[(2~{R},3~{S},4~{S},5~{R})-3,4-bis(oxidanyl)-5-[3-[4-[[(phenylmethyl)carbamoylamino]methyl]-1,2,3-triazol-1-yl]propyl]oxan-2-yl]methyl ~{N}-[(2~{S})-2-azanyl-4-methyl-pentanoyl]sulfamate | C26 H41 N7 O8 S | 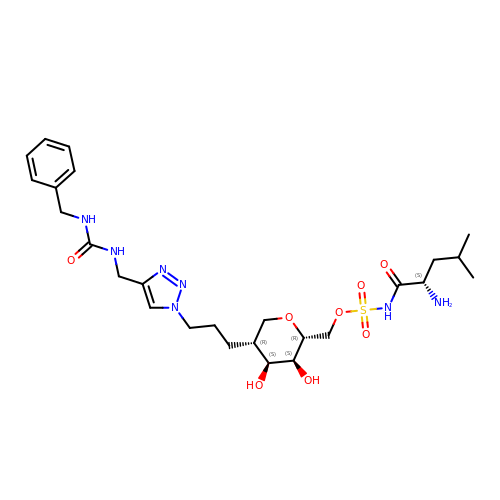BUJGEMBLEXNUBK-MENZVKOBSA-N>MSQAEFEKAAEEVRHLKTKPSDEEMLFIYGHYKQATVGDINTERPGMLDFTGKAKWDAWNELKGTSKEDA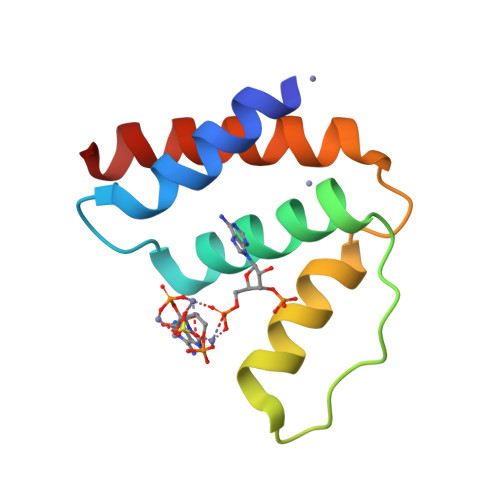MKAYINKVEELKKKYGI[2x]OCTANOYL-COENZYME A | C29 H50 N7 O17 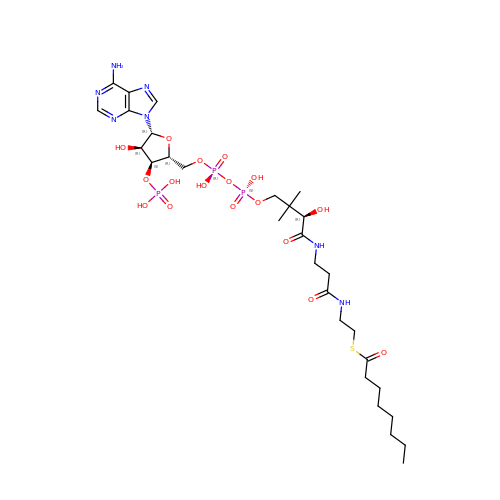P3 S | KQMZYOXOBSXMII-CECATXLMSA-N>ADGKYAQKLFNDLFEDYSNALRPVEDTDKV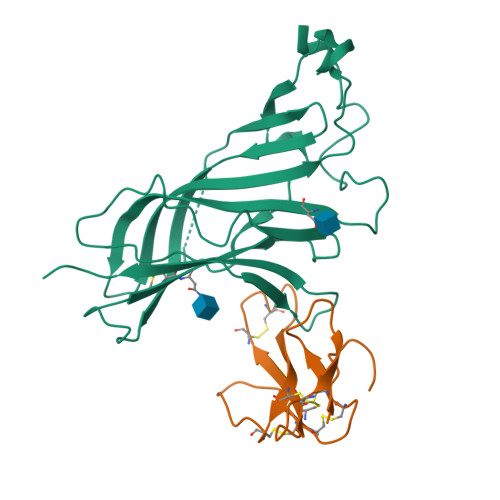LNVTLQITLSQIKDMDERNQILTAYLWIRQIWHDAYLTWDRDQYDGLDSIRIPSDLVWRPDIVLYNKADDESSEPVNTNVVLRYDGLITWDAPAITKSSCVVDVTYFPFDNQQCNLTFGSWTYNGNQVDIFNALDSGDLSDFIEDVEWEVHGMPAVKNVISYGCCSEPYPDVTFTLLLKRRSHHHHHH[2x];>[2x]IVCHTTATSPISAVTCPPGENLCYRKMWCDVFCSSRGKVVELGCAATCPSKKPYEEVTCCSTDKCNPHPKQRPG The alkylation of deoxyguanosine in DNA at the O6 position, exemplified by exposure to N-benzylmethylnitrosamine and the formation of O6-benzyl-2′-deoxyguanosine nucleoside (O6-Bn-dG), is cytotoxic and mutagenic. The O6-Bn-dG lesion is representative of bulky DNA adducts involved in the initiation of gene mutations. Analyses of DNA containing O6-Bn-dG or dPer paired opposite each other or natural bases have demonstrated that the O6-Bn-dG:dPer pair is more stable than any pairing of the damaged base opposite any natural base, or of dPer opposite a natural base. Herein, we explain the molecular basis by which dPer distinguishes between O6-Bn-dG and dG.

When deoxyguanosine at position G4 of the Dickerson–Drew dodecamer (DDD) was replaced by O6-Bn-dG, and deoxycytosine C9 was replaced with dPer to form the modified O6-Bn-dG:dPer (DDD-XY) duplex [5′-d(C1G2C3X4A5A6T7T8Y9G10C11G12)-3′]2 (X = O6-Bn-dG, Y = dPer), dPer intercalated into the duplex and adopted the syn conformation about the glycosyl bond. This provides a binding pocket that allows the benzyl group of O6-Bn-dG to intercalate between Per and thymine of the 3′-neighbor A:T base pair. A second crystal, crystallized from the buffer containing 80 mM SrCl2, diffracted at the greater resolution of 1.7 Å, also in space group P212121 (orthorhombic). The data from the second crystal were phased using molecular replacement methods in which the structure from the first crystal was used as a starting model. One Sr2+ ion was identified in the electron density map based on its low B-factor and the characteristic geometry, as well as one spermine. Although no electron density was observed for the 5′-terminal bases C1 and C13, and thus their positions could not be determined with certainty, the 3′-terminal bases G12 and G24 rotated out of the duplex toward the major groove of adjacent molecules. The simultaneous insertion of both dPer and the benzyl ring of the O6-Bn-dG base increased the helical rise between neighboring base pairs C3:G22 and A5:T20 to 9.5 Å, as compared with the anticipated rise of ∼6.8 Å in B-DNA. In the crystallographic data obtained at a resolution of 1.7 Å, when inserted into the electron density map in the syn conformation, the resulting crystallographic R factor was minimized. If dPer was instead inserted into the electron density map in the anti conformation, it did not fit well, and residual difference (Fo-Fc) Fourier electron density was observed. The data suggest that in this DNA sequence the presence of dPer ‘traps’ the benzyl ring of O6-Bn-dG between the dPer nucleotide and T20, providing a mechanism whereby dPer recognizes the O6-Bn-dG DNA damage.

>[2x]CGCNAATTXGCG>[2x]MHHHHHHMKFTVEREHLLKPLQQVSGPLGGRPTLPILGNLLLQVADGTLSLTGTDLEMEMVARVALVQPHEPGATTVPAR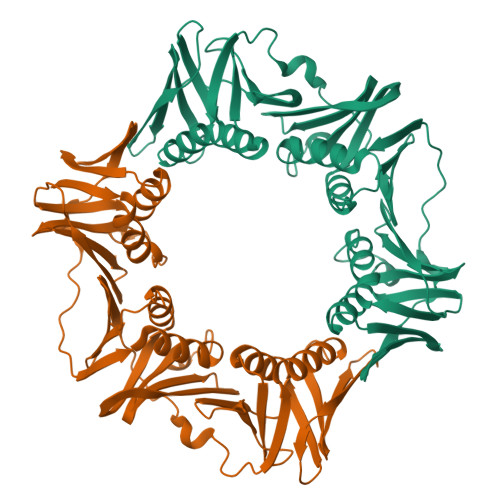KFFDICRGLPEGAEIAVQLEGERMLVRSGRSRFSLSTLPAADFPNLDDWQSEVEFTLPQATMKRLIEATQFSMAHQDVRYYLNCMLFETEGEELRTVATDGHRLAVCSMPIGQSLPSHSVIVPRKGVIELMRMLDGGDNPLRVQIGSNNIRAHVGDFIFTSKLVDGRFPDYRRVLPKNPDKHLEAGCDLLKQAFARAAILSNEKFRGVRLYVSENQLKITANNPEQEEAEEILDVTYSGAEMEIGFNVSYVLDVLNALKCENVRMMLTDSVSSVQIEDAASQSAAYVVMPMRL>MGSSHHHHHHSSGLVPRGSHSNYGKSADGTVTIEYFNQKKEMTKTLEEITRDFEKENPKIKVKVVNVPNAGEVLKTRVLAGDVPDVVNIYPQSIELQEWAKAGVFEDLSNKDYLKRVKNGYAEKYAVNEKVYNVPFTANAYGIYYNKDKFEELGLKVPETWDEFEQLVKDIVAKGQTPFGIAGADAWTLNGYNQLAFATATGGGKEANQYLRYSQPNAIKLSDPIMKDDIKVMDILRINGSKQKNWEGAGYTDVIGAFARGDVLMTPNGSWAITAINEQKPNFKIGTFMIPGKEKGQSLTVGAGDLAWSISATTKHPKEANAFVEYMTRPEVMQKYYDVDGSPTAIEGVKQAGEDSPLAGMTEYAFTDRHLVWLQQYWTSEADFHTLTMNYVLTGDKQGMVNDLNAFFNPMKAD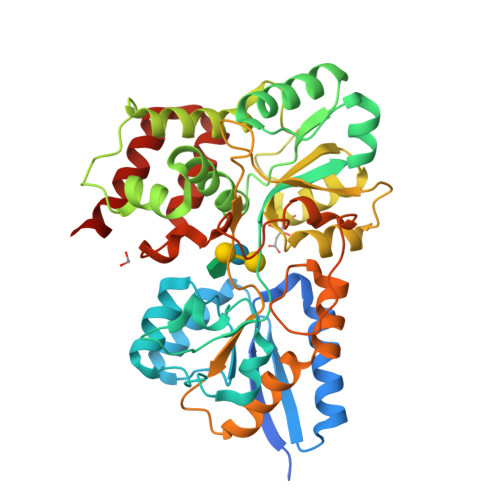VD[2x]>HMEMDKRMKSLAMTAFFGELSTLDIMALIMSIFKRHPNNTIFSVDKDGQFMIDFEYDNYKASQYLDLTLTPISGDECKTHASSIAEQLASVDIIK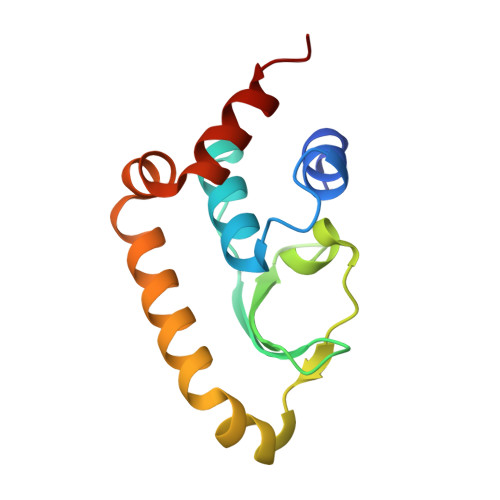EDISEYIKTTPRLKRFIKKYRNRS[2x]> SN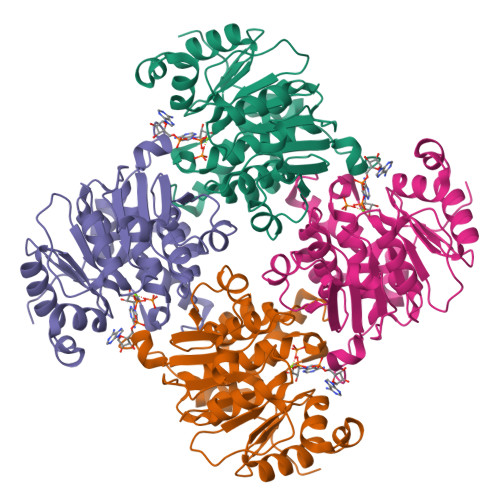AMNVPFWTEEHVRATLPERDAESHKGTYGTALLLAGSDDMPGAALLAGLGAMRSGLGKLVIGTSENVIPLIVPVLPEATYWRDGWKKAADAQLEETYRAIAIGPGLPQTESVQQAVDHVLTADCPVILDAGALAKRTYPKREGPVILTPHPGEFFRMTGVPVNELQKKRAEYAKEWAAQLQTVIVLKGNQTVIAFPDGDCWLNPTGNGALAKGGTGDTLTGMILGMLCCHEDPKHAVLNAVYLHGACAELWTDEHSAHTLLAHELSDILPRVWKRFE> GDRVADVIESSIGDSVSRALTHALPAPTGQDTQVSSHRLDTGKVPALQAAEIGASSNASDESMIETRCVLNSHSTAETTLDSFFSRAGLVGEIDLPLKGTTNPNGYANWDIDITGYAQMRRKVELFTYMRFDAEFTFVACTPTGEVVPQLLQYMFVPPGAPKPDSRESLAWQTATNPSVFVKLSDPPAQVSVPFMSPASAYQWFYDGYPTFGEHKQEKDLEYGA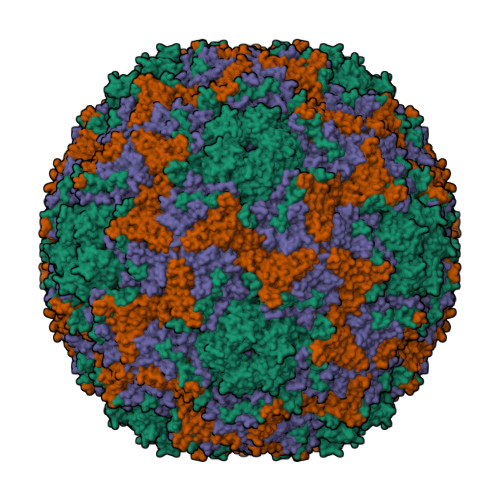CPNNMMGTFSVRTVGTSKSKYPLVVRIYMRMKHVRAWIPRPMRNQNYLFKANPNYAGNSIKPTGTSRTAITTL;> SPSAEACGYSDRVAQLTIGNSTITTQEAANIIVGYGEWPSYCSDSDATAVDKPTRPDVSVNRFYTLDTKLWEKSSKGWYWKFPDVLTETGVFGQNAQFHYLYRSGFCIHVQCNASKFHQGALLVAVLPEYVIGTVAGGTGTEDSHPPYKQTQPGADGFELQHPYVLDAGIPISQLTVCPHQWINLRTNNCATIIVPYINALPFDSALNHCNFGLLVVPISPLDYDQGATPVIPITITLAPMCSEFAGLRQAVTQ;> GFPTELKPGTNQFLTTDDGVSAPILPNFHPTPCIHIPGEVRNLLELCQVETILEVNNVPTNATSLMERLRFPVSAQAGKGELCAVFRADPGRNGPWQSTLLGQLCGYYTQWSGSLEVTFMFTGSFMATGKMLIAYTPPGGPLPKDRATAMLGTHVIWDFGLQSSVTLVIPWISNTHYRAHARDGVFDYYTTGLVSIWYQTNYVVPIGAPNTAYIIALAAAQKNFTMKLCKDASDILQTGTIQ;> MGSQVSTQRSGSHENSNSATEGSTINYTTINYYKDSYAATAGKQSLKQDPDKFANPVKDIFTEMAAPLK>[2x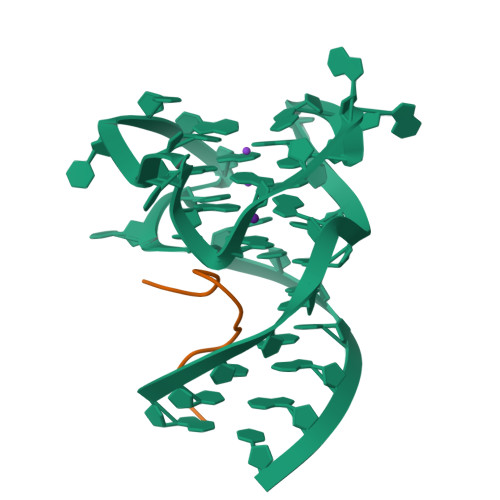]ARGDGRRRGGGGRGQGGR>[2x]MSLSFLKHVQDCNTHDLSNFVRFVIEGRRVGWVRKALAQRLKAHGRVFDVTRDAVLLSASLRTPQSRTRAVADVVDRLADEGVVPAPRGELYRVNQSWGEPTL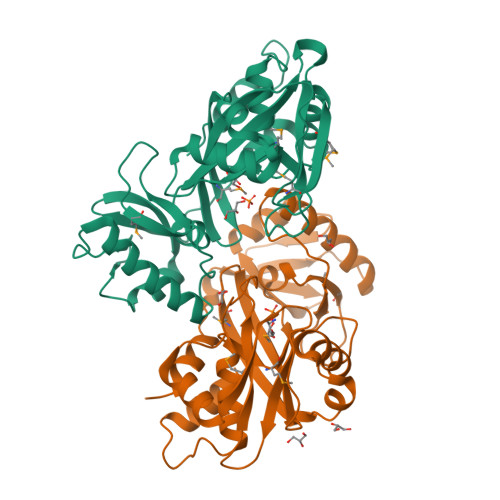MLLDRAVVPTFGVRAYGVHLNGYVGAGADLHLWIGRRSPDKSVAPGKLDNMVAGGQPADLSLRQNLIKECAEEADLPEALARQAIPVGAITYCMESPAGIKPDTLFLYDLALPEDFRPHNTDGEMADFMLWPAAKVVEAVRTTEAFKFNVNLTVIDFAIRHGLIDPDNEPDYQEILAGLRGRPRERAASEGHHHHHH> MPKIKSFAPAWLNEPAPGHKLFAPAADDGTATVPLAYGKKIKPGPRRTIARRGTEIFVACGKQIRWGDLAQLKESWESRPSRSSVGPTSTKKDSSDFDDGAATAGYRIIKTPVADDIRQLVMSPNQDFLAVLTSHTVHICILPDSSHLHIQDTTPFKPKFWTLGPTTHVTSRSAVVSAVWHPLGVNGHALVTVTEDAIVRVWELSTADRWTFDAPTLAIDLKKLADATYLDQDFGVSTSATNKGFSPDAFDMEVAAACFPTRDSGGWAPMTLWLAMTSGDVYALCPLLPQRWTPPPTLIPSLSASIVAKVAAAEDNPESTPEERLVAQQQLEWM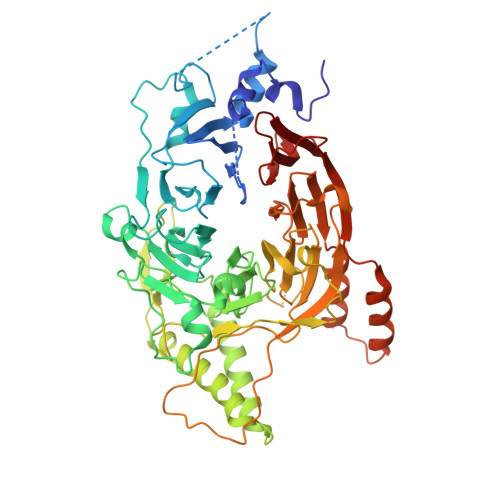SEIDNQEPKLVEEATGEATIEVYTRPSRPGLVPKLQGPFDFDLNPEDEQDDEVELKDIYVIGEKPRVADLMRGEEEELEMMKEDQHNGLSLNIICLLSTSGQVKICLDIDGVEAQWLPPRSKNKRLFAPPPEPPSLLTFQTFDTLKPAEVTPDGWPMFSEDATSPYSFYVTHPAGITYISLTPWVFRLESELQSDSEAGTEFRIDLLAKGQGSERDRIFTQTRTQSPLAAATSIDDPDLGYFILSATQTDPIALFFETPER> PPLA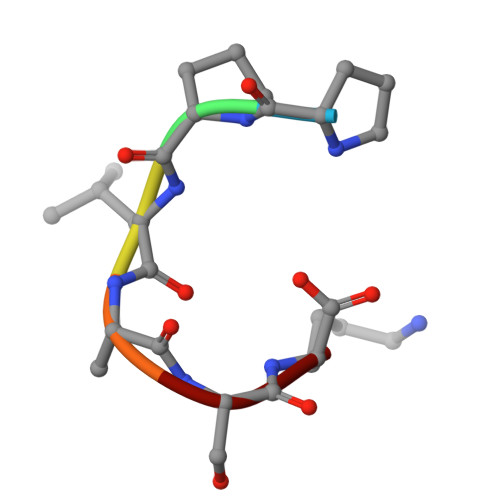SK Here, we determine the high-resolution structures of cyclic di-pyrimidine-synthesizing cGAS/DncV-like nucleotidyltransferases (CD-NTases) in clade E (CdnE) in its apo, substrate-, and intermediate-bound states. CD-NTases share an N-terminal core domain with templated and non-templated polymerases of the nucleotidyltransferase (NTase) superfamily, but the C-terminal helical domain shows a higher degree of variation. Three conserved acidic residues in the central β-sheet of the NTase domain coordinate with two metal ions (A and B) that are essential for catalysis. Based on sequence conservation and structural similarity, it is proposed that the cyclic di-pyrimidine-synthesizing CdnE proteins, including ClCdnE, EfCdnE, and LpCdnE, form smaller donor pockets that act as molecular gauges to recognize and retain the binding of pyrimidine nucleotides but weaken or exclude the binding to purine nucleotides.

The native structure of EfCdnE was determined to be a 1.75-Å resolution. When compared with ClCdnE, helix α2 of EfCdnE was shorter by one turn at the N-terminus. The overall root-mean-square deviation (RMSD) is 1.38 Å between 280 matched pairs of Cα atoms. Other significant deviations were observed in the βB’-α3 loop, βD-βE loop, βE-βF loop, and α7-α8 loop. Despite the differences in local regions, the dispositions of the NTase and helical domains were similar in the native structures of ClCdnE, EfCdnE, and LpCdnE, respectively. Similarly, the side chains of Glu267 and Arg279 in EfCdnE are engaged in salt-bridging interactions and would have substantial clashes with the donor base if it were a purine nucleotide. This observation explains why we could not detect the binding of ATP and GTP analogs to EfCdnE in the ITC experiments.

> MSKFSESTLSGWTKPASVTEEDRIENTISMIKSAIKNDNNFDNLVYEVFVQGSYGNNTNVRTNSDIDVNIMLTSTFYSKYPEGKTNSDYGFTDGTITYNEYKNLILTALTNKFGTGNVTVGNKSIKITSNSYRVEADCIPSLLYRNYEYENSSSPNNYIEGIKYFASDNTSVVNYPKVHINNGIEKNNQTHKNYKRLVRVIKRLRNKMTAENHFTNENITSFLIECLIWNVPNNYINDYDTWDETIKQTLIFIKSSINDNSYKNWTEVSGMFYLFHNNRKWTSDDVSSFVNSLWSFMEYLEHHHHHH>[10x]MGSSHHHHHHSQDPENLYFQGSAANADFELFRVFLEKTCGIVLGSNKQYLVSSRLNKLMEQQGIKSLGELVQRIQTQRGGLREMVVDAMTTNETLWFRDTYPFEVLKQRVLPELIKANGGQRLRIWSAACSSGQEPYSLSMAIDEFEK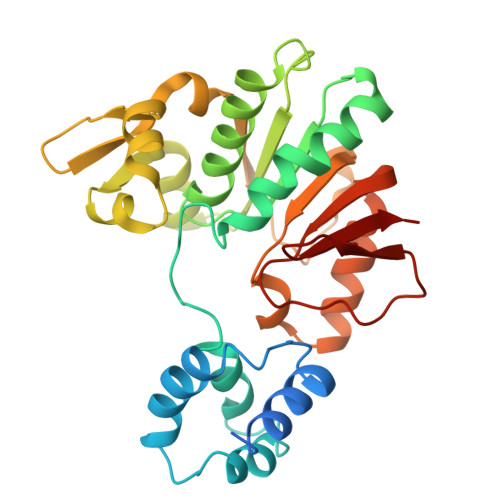TNLGQLKAGVQIVATDLSGSMLTAAKAGEYDTLAMGRGLSPERLQRYFDAKGPGRWAVKPAIRSRVEFRALNLLDSYASLGKFDMVFCRNVLIYFSAEVKRDILLRIHGTLKPGGYLFLGASEALNNLPDHYQMVQCSPGIIYRAK>[8x]MLAMSPPKPAVELDRHIDLDQAHAVASGGARIVLAPPARDRCRASEARLGAVIREARHVYGLTTGFGPLANRLISGENVRTLQANLVHHLASGVGPVLDWTTARAMVLARLVSIAQGASGASEGTIARLIDLLNSELAPAVPSRGTV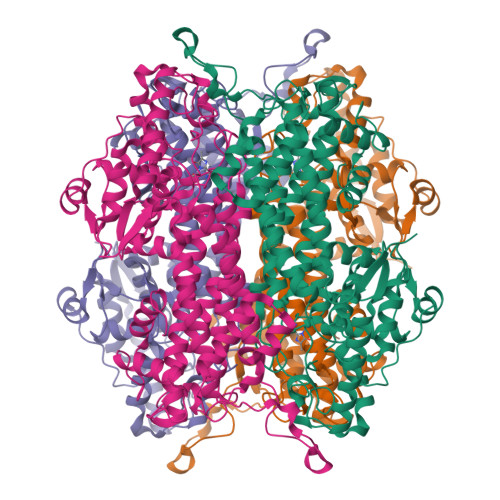GASGDLTPLAHMVLCLQGRGDFLDRDGTRLDGAEGLRRGRLQPLDLSHRDALALVNGTSAMTGIALVNAHACRHLGNWAVALTALLAECLRGRTEAWAAALSDLRPHPGQKDAAARLRARVDGSARVVRHVIAERRLDAGDIGTEPEAGQDAYSLRCAPQVLGAGFDTLAWHDRVLTIELNAVTDNPVFPPDGSVPALHGGNFMGQHVALTSDALATAVTVLAGLAERQIARLTDERLNRGLPPFLHRGPAGLNSGFMGAQVTATALLAEMRATGPASIHSISTNAANQDVVSLGTIAARLCREKIDRWAEILAILALCLAQAAELRCGSGLDGVSPAGKKLVQALREQFPPLETDRPLGQEIAALATHLLQQSPV Abortive infection (Abi) is a bacterial antiphage defense strategy involving suicide of the infected cell. Some Abi pathways involve polymerases that are related to reverse transcriptases. They are unique in the way they combine the ability to synthesize DNA in a template-independent manner with protein priming. Here, we report crystal and cryo-electron microscopy structures of two Abi polymerases: AbiK and Abi-P2. Both proteins adopt a bilobal structure with an RT-like domain that comprises palm and fingers subdomains and a unique helical domain.

To test this assumption, we have prepared a Ll-AbiK variant in which Tyr44 is substituted with phenylalanine. This protein was unable to catalyze protein-primed DNA synthesis (see below), so we assumed that its structure would reveal the conformational state before nucleic acid polymerization starts. The structure of Ll-AbiK Y44F was determined at 2.7 Å resolution by cryo-EM and it is essentially identical to that of the wild-type enzyme except for a fragment of the 21–57 loop. Residues 32–42 could not be traced in the Ll-AbiK Y44F structure implying a higher mobility and/or conformational heterogeneity of this region. The fragment spanning residues 43–49, which in the wild-type Ll-AbiK–DNA adduct structure runs parallel to the nucleic acid chain, adopts a different trajectory and runs toward the DNA-binding cleft. As a result the location of the C-α of Tyr/Phe44 changes by 15 Å positioning this residue in the vicinity of the polymerase active site. This conformation very likely resembles the state in which the protein attaches the first nucleotide to the side chain of Tyr44. Nevertheless, the structure of Y44F variant reveals that a conformational change of the loop harboring the key tyrosine, which can position it for the protein priming at the active site, can be readily accommodated in the overall hexameric architecture of the enzyme. As expected, replacement of the protein-priming tyrosine with phenylalanine (Y44F) inactivated the enzyme, confirming the essential role of the hydroxyl group of Tyr44 in DNA synthesis. Similarly, cryo-EM analysis of the other inactive mutant, Y44F, showed that the majority of the particles were monomers and only a fraction of them, which was used for structure determination, corresponded to hexamers.

>[6x]GSMKKEFTELYDFIFDPIFLVRYGYYDRSIKNKKMNTAKVELDNEFGKSDSFYFKVFNMESFADYLRSHDLKTHFNGKKPLSTDPVYFNIPKNIEARRQYKMPNLYSYMALNYYICDNKKEFIEVFIDNKFSTSKFFNQLNFDYPKTQEITQTLLYGGIKKLHLDLSNFYHTLYTHSIPWMIDGKSASKQNRKKGFSNTLDTLITACQYDETHGIPTGNLLSRIITELYMCHFDKQMEYKKFVYSRYVDDFIFPFTFENEKQEFLNEFNLICRENNLIINDNKTKVDNFPFVDKSSKSDIFSFFENITSTNSNDKWIKEISNFIDYCVNEEHLGNKGAIKCIFPVITNTLKQKKVDTKNIDNIFSKRNMVTNFNVFEKILDLSLKDSRLTNKFLTFFENINEFGFSSLSASNIVKKYFSNNSKGLKEKIDHYRKNNFNQELYQILLYMVVFEIDDLLNQEELLNLIDLNIDDYSLILGTILYLKNSSYKLEKLLKKIDQLFINTHANYDVKTSRMAEKLWLFRYFFYFLNCKNIFSQKEINSYCQSQNYNSGQNGYQTELNWNYIKGQGKDLRANNFFNELIVKEVWLISCGENEDFKYLN>PSVYDAAAQLTADVKKDLRDSWKVIGSDK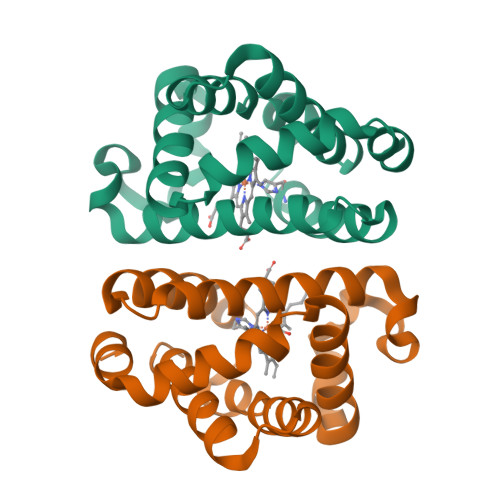KGNGVALMTTLFADNQETIGYFKRLGDVSQGMANDKLRGHSIGLMYALQNFIDQLDNPDDLVCVVEKFAVNHITRKISAAEFGKINGPIKKVLASKNFGDKYANAWAKLVAVVQAAL[2x]2-({2-[(4-carbamoylphenyl)amino]pyrimidin-4-yl}amino)benzamide | C18 H16 N6 O2 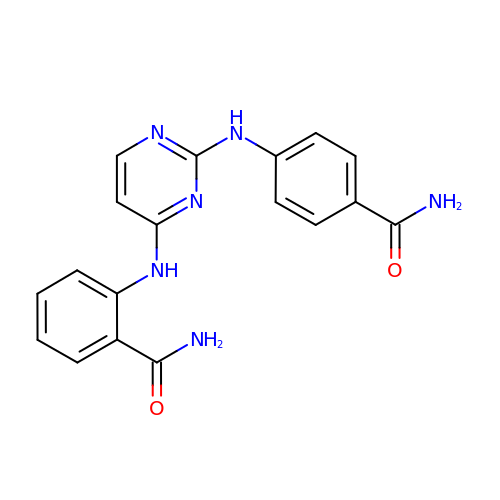| DYZNHQCKJOEZRJ-UHFFFAOYSA-N> MMRCSRGCRRQLRPYYNLPSKSDHGRKMTGFLTPYRHWMWKQNELWRNVHEAQFEHLRKVYKRQWLESFRVNADEYIYKYNITKAAQLAQWEYEMQAQEKKRLEAKQMTEGRQALKKKHLDLLREFHERQFFFWYERASERLQSMNLIQYIPQSRVQEHIERELDKYVAGKSEAYPLNFVGQMPLVEDREGNIVEVPEGLLTNHVSEHPESTVKPHQPHESTSVSVEEQLLRTMASAREESLEEWIDDSRALSETI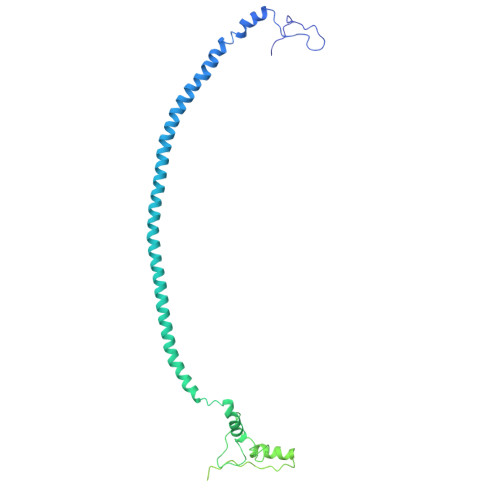DDISREEEQRDEDTRVARSMEETDNEREISRRMYIDRGKTGSKAIFRRPTLSETDGGSASIPVGGVAASPADTSAPMRRRKKGKLDKAHALQEQQDAMIARMSAKSLKDGESSISIVKRGEIATSRGRIRDKAAIPTQEVLMQKPELAAGSVPNARISFKDKVDQLYHRGKYKQKKEDDNNPNEDL> GQLAPGITMSEIDRIAQNIIKSHLETCQYTMEELHQLAWQTHTYEEIKAYQSKSREALWQQCAIQITHAIQYVVEFAKRITGFMELCQNDQILLLKSGCLEVVLVRMCRAFNPLNNTVLFEGKYGGMQMFKALGSDDLVNEAFDFAKNLCSLQLTEEEIALFSSAVLISPDRAWLLEPRKVQK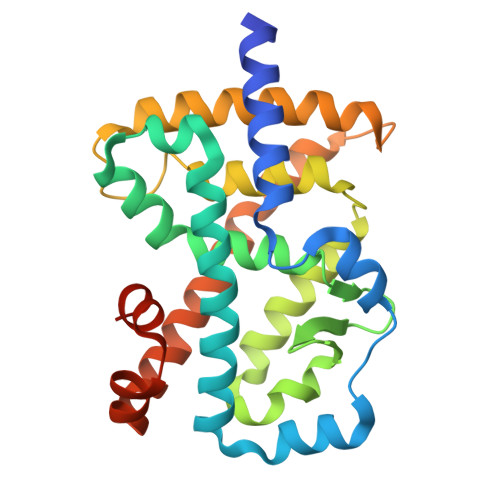LQEKIYFALQHVIQKNHLDDETLAKLIAKIPTITAVCNLHGEKLQVFKQSHPDIVNTLFPPLYKELFNPDCAAVCK> GSSGSSGMANERMNLMNMAKLSIKGLIESALNLGRTLDSDYAPLQQFFVVMEHCLKHGLKAKKTFLGQNKSFWGPLELVEKLVPEAAEITASVKDLPGLKTPVGRGRAWLRLALMQKKLSEYMKALINKKELLSEFYEVNALMMEEEGAIIAGLLVGLNVIDANFCMKGEDLDSQVGVIDFSMYL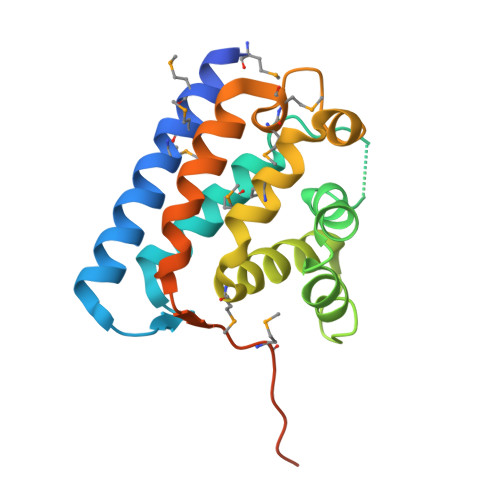KDGNS> MSRSKRDNNFYSVEIGDSTFTVLKRYQNLKPIGSGAQGIVCAAYDAILERNVAIKKLSRPFQNQTHAKRAYRELVLMKCVNHKNIIGLLNVFTPQKSLEEFQDVYIVMELMDANLCQVIQMELDHERMSYLLYQMLCGIKHLHSAGIIHRDLKPSNIVVKSDCTLKILDFGLARTAGTSFMMTPYVVTRYYRAPEVILGMGYKENVDIWSVGCIMGEMIKGGVLFPGTDHIDQWNKVIEQLGTPSPEFMKKLQPTVRTYVENRPKYAGYSFEKLFPDVLFPADSEHNKLKASQARDLLSKMLVIDASKRISVDEALQHPYINVWYDPSEAEAPPPKIPDKQLDEREHTIEEWKELIYKEVMDLEH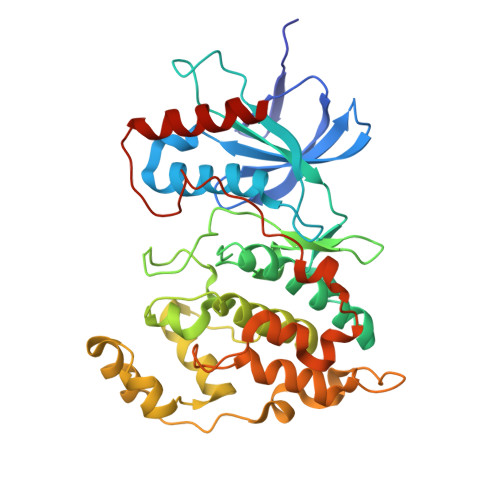HHHHH> MTLSIENQNKLDEFWAYCVKNQYFNIGYPESADFDYTILERFMRFSINNCGDWAEYSNYLLNSFDFEKEVMEYFADLFKIPFEDSWGYVTNGGTESNMFGVYLGRELFPDGTLYYSKDTHYSVAKI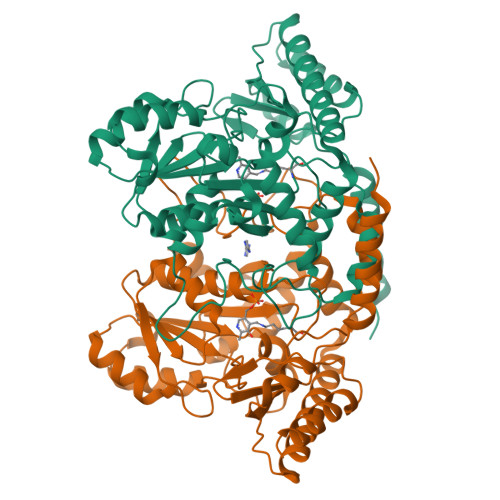VKLLRIKSQLVDSLPNGEIDYDDLISKIKQDDEKHPIIFANIGTTVRGAIDDISKIQAMIGELGIKREDYYIHADAALSGMILPFVDEPQGFNFADGIDSIGVSGHKMIGSPIPCGIVVAKKRNVDAISVEIDYISAHDKTITGSRNGHTPLMMWVAVKSHSHADFKRRINRSLDLAQHAVQRLQTAGINAWCNKNSITVVFPCPSEAVWKKHCLATSGGQAHLITTAHHLDASKVDALIDDVIKDAN> HHHHHHAPAFRYTRSQSFDIFDINQKCFVLESPTQLVALHLQGPSSSQKVRLNIALYRPRGPRGSAGTGQMPVALGIKGYKLYMS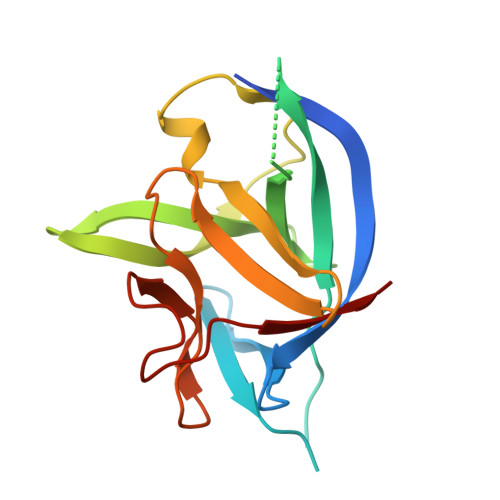CVMSGTEPTLQLEEADVMRDIDSVELTRFIFYRLDSPTEGTTRFESAAFPGWFICTSLQPAQPVGITNQPDQVNIATYKLSGR>[2x]SSANEDMPVERILEAELAVEPKTETYVEANMGLNPSSPNDPVTNICQAADKQLFTLVEWAKRIPHFSELPLD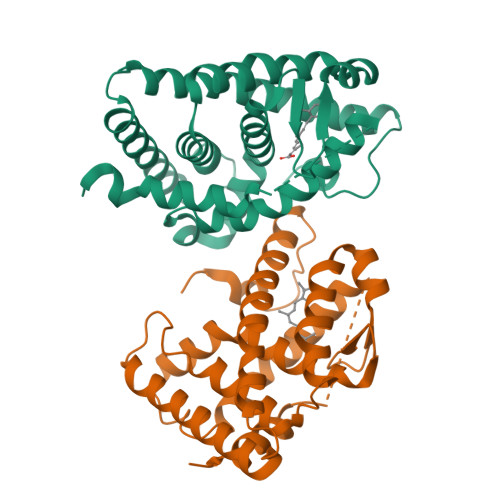DQVILLRAGWNELLIASFSHRSIAVKDGILLATGLHVHRNSAHSAGVGAIFDRVLTELVSKMRDMQMDKTELGCLRAIVLFNPDSKGLSNPAEVEALREKVYASLEAYCKHKYPEQPGRFAKLLLRLPALRSIGLKCLEHLFFFKLIGDTPIDTFLMEMLEAPHQMT>[2x]MSPFPLTSMDKAFITVLEMTPVLGTEIINYRDGMGRVLAQDVYAKDNLPPFPASVKDGYAVRAADGPGDRFIIGE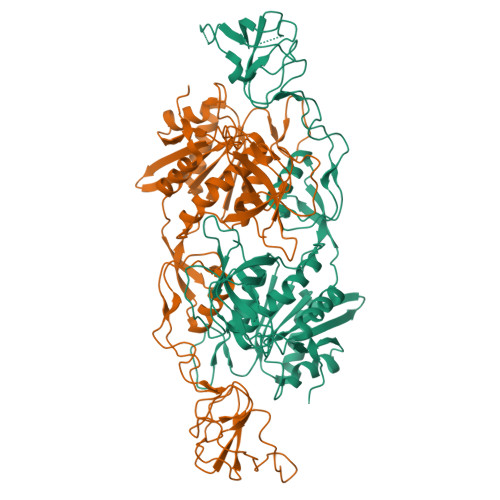SQAGEQPTQTVMPGQVMRVTTGAPIPCGADAVVQVEDTELIRESDDGTEELEVRILVQARPGQDIRPIGHDIKRGECVLAKGTHMGPSEIGLLATVGVTEVEVNKFPVVAVMSTGNELLNPEDDLLPGKIRDSNRSTLLATIQEHGYPTINLGIVGDNPDDLLNALNEGISRADVIITSGGVSMGEKDYLKQVLDIDLHAQIHFGRVFMKPGLPTTFATLDIDGVRKIIFALPGNPVSAVVTCNLFVVPALRKMQGILDPRPTIIKARLSCDVKLDPRPEYHRCILTWHHQEPLPWAQSTGNQMSSRLMSMRSANGLLMLPPKTEQYVELHKGEVVDVMVIGRL>[2x]IGGNFGVQPVVESTPTAYPVTFKSKDVPTPPPAGSSVETTPVNRPAVGAAMRLPRRNIASYKQDGTEIPDKHQAEEHLPLKEKDILFLDGTLKEQADKLKKKINERYSDVRVITSKKEEEKYQYQFVRAGYVFTRAEGKDNEKEKTSDGKEFVNRFSYDGFVYYSGERPSQSLPSAGT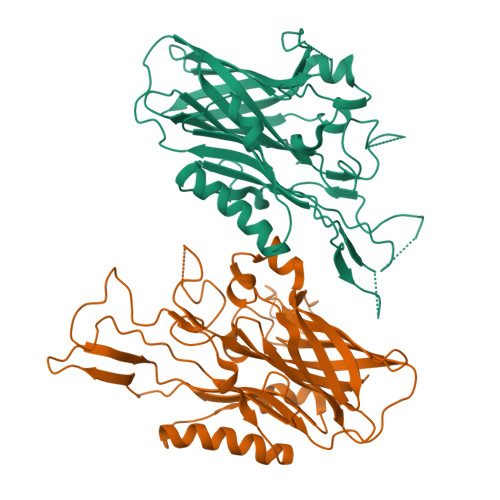VQYSGNWQYMTDAKRHRTGKAVSSTDLGYTTYYGNEIGATSYEARDADDREKHPAEYTVDFDNKTLNGKLIKNQYVQNKSNPNEPKKPLTIYDITATLDGNRFTGSAKVSTEVKTQHADKEYLFFHTDADQRLEGGFFGDNGEELAGRFISNDNSVFGVFAGKQKTET> MFIQEPKKLIDTGEIGNASTGDILFDGGNKINSDFNAIYNAFGDQRKMAVANGTGADGQIIHATGYYQKHSITEYATPVKVGTRHDIDTST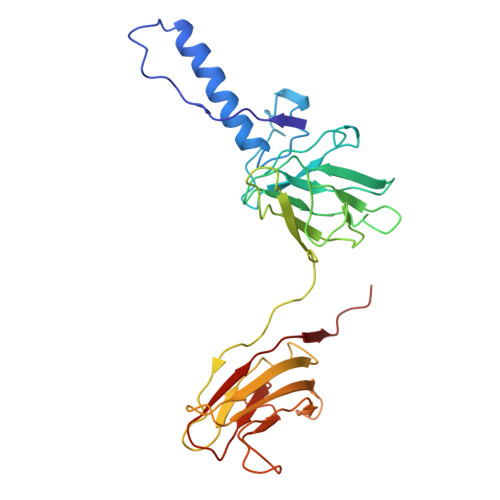VGVKVIIERGELGDCVEFINSNGSISVTNPLTIQAIDSIKGVSGNLVVTSPYSKVTLRCISSDNSTSVWNYSIESMFGQKESPAEGTWNISTSGSVDIPLFHRTEYNMAKLLVTCQSVDGRKIKTAEINILVDTVNSEVISSEYAVMRVGNETEEDEIANIAFSIKENYVTATISSSTVGMRAAVKVIATQKIGVAQ> VVTYTTLIDGLAKAGRLEEALQLFQEMKEKGVKPDVVTYTTLID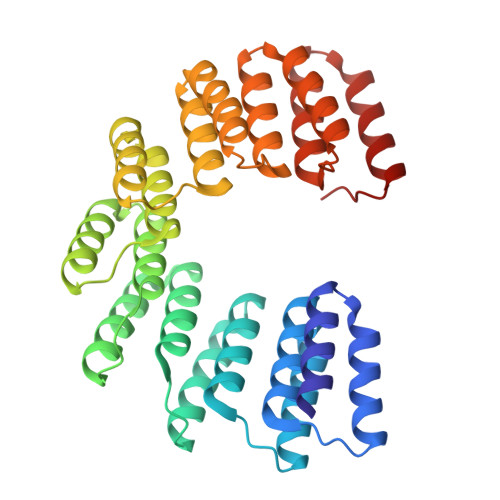GLAKAGRLEEALQLFQEMKEKGVKPDVVTYTTLIDGLAKAGRLEEALQLFQEMKEKGVKPDVVTYTTLIDGLAKAGRLEEALQLFQEMKEKGVKPDVVTYTTLIDGLAKAGRLEEALQLFEEMKEKGVKPDVVTYTTLIDGLAKAGRLEEALQLFQEMKEKGVKPDVVTYTTLIDGLAKAGRLEEALQLFEEMKEKGVKPDVVTYTTLIDGLAKAGRLEEALQLFEEMKEKGVKPDVVTYTTLIDGLAKAGRLEEALQLFQEMKEKGVKPD> MGSSHHHHHHSSGRENLYFQGMTTAKRDTYTPETLLSVAVQVFIERGYDGTSMEHLSKAAGISKSSIYHHVTGKEELLRRAVSRALDELFGILDEEHARVGTAAERLEYVVRRMVEVLMAELPYVTLLLRVRGNTGTERWALERRREFDHRVAALLKDAAAEGDVRADVEVRLATRLV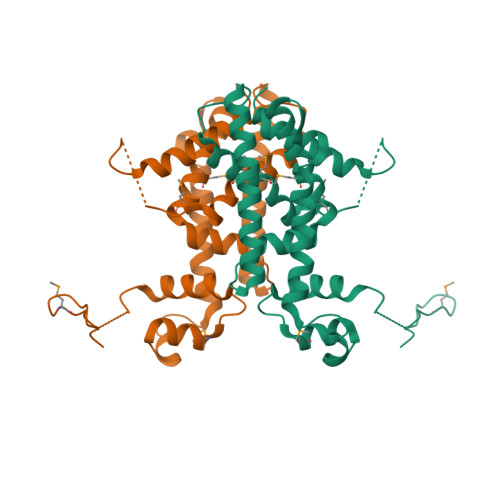FGMINSIVEWYRPEGPDGRSDASGASGVSGAGEREVVDAVARLVFGGLRKAS> MSQEQYTENLKVIVAEKLAGIP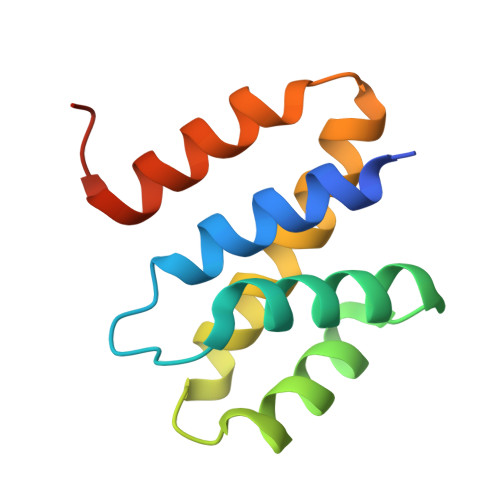NFNEDIKYVAEYIVLLIVNGGTVESVVDELASLFDSVSRDTLANVVQTAFFALEALQQGESAENIVSKIRMMNAQSLGQSDIA[2-(1,3-benzodioxol-5-ylamino)-1,3-thiazol-4-yl]-[(3R,5S)-3,5-dimethylpiperidin-1-yl]methanone 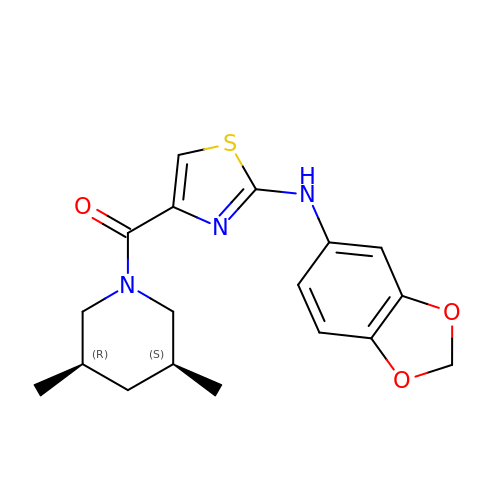| C18 H21 N3 O3 S | UBMOUBBRNPNZPM-TXEJJXNPSA-N> MSQRITIDPVTRIEGHLRIDCEIENGVVSKAWASGTMWRGMEEIVKNRDPRDAWMIVQRICGVCTTTHALSSVRAAESALNIDVPVNAQYIRNIILAAHTTHDHIVHFY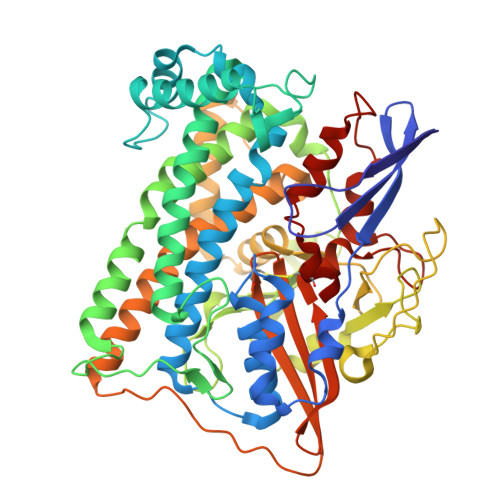QLSALDWVDITSALQADPTKASEMLKGVSTWHLNSPEEFTKVQNKIKDLVASGQLGIFANGYWGHPAMKLPPEVNLIAVAHYLQALECQRDANRVVALLGGKTPHIQNLAVGGVANPINLDGLGVLNLERLMYIKSFIDKLSDFVEQVYKVDTAVIAAFYPEWLTRGKGAVNYLSVPEFPTDSKNGSFLFPGGYIENADLSSYRPITSHSDEYLIKGIQESAKHSWYKDEAPQAPWEGTTIPAYDGWSDDGKYSWVKSPTFYGKTVEVGPLANMLVKLAAGRESTQNKLNEIVAIYQKLTGNTLEVAQLHSTLGRIIGRTVHCCELQDILQNQYSALITNIGKGDHTTFVKPNIPATGEFKGVGFLEAPRGMLSHWMVIKDGIISNYQAVVPSTWNSGPRNFNDDVGPYEQSLVGTPVADPNKPLEVVRTIHSFDPCMACAVH>FLGNDTVEIKDGRFFIDGYDAIELAEKFGTPLYVMSEEQIKINYNRYIEAFKRWEEETGKEFIVAYAYKANANLAITRLLAKLGCGADVVSGGELYIAKLSNVPSKKIVFNGNCKTKEEIIMGIEANIRAFNVDSISELILINETAKELGETANVAFRINPNVNPKTHPKISTGLKKNKFGLDVESGIAMKAIKMALEMEYVNVVGVHCHIGSQLTDISPFIEETRKVMDFVVELKEEGIEIEDVNLGGGLGIPYYKDKQIPTQKDLADAIINTMLKYKDKVEMPN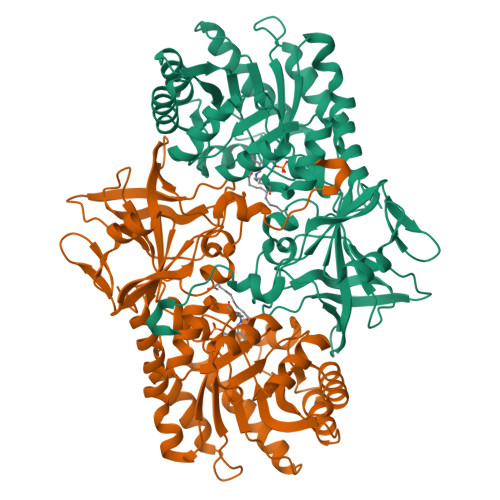LILEPGRSLVATAGYLLGKVHHIKETPVTKWVMIDAGMNDMMRPAMYEAYHHIINCKVKNEKEVVSIAGGLCESSDVFGRDRELDKVEVGDVLAIFDVGAYGISMANNYNARGRPRMVLTSKKGVFLIRERETYADLIAKDIVPPHLL[2x]> PDCGVICENGKCVVKENGSNCRHYNIYEPAPDVKTTEINVIVSGDEQGIITKKLQDFCMNPNNENGTNNQIWKCYYKDEKEDKCKVETKSGNSTYKEKITSFDEFFDFWVRKLLIDTIKWETELTYCINNTTNADCNNECNKNCVCFDKWVKQKEKEWKNIMDLFTN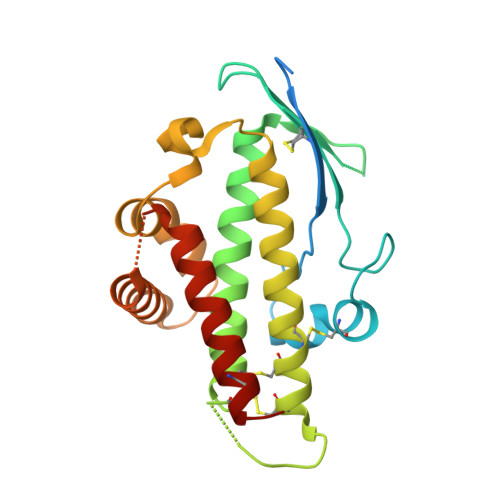KHDIPKKYYLNINDLFNSFFFQVIYKFNEGEAKWNKLKENLKKKTESSKKNKGTKDSEAAIKVLFDHLKETATICKDNNTNEAC> MVPISPIETVPVKLKPGMDGPKVKQWPLTEEKIKALVEICTEMEKEGKISKIGPENPYNTPVFAIKKKDSTKWRKLVDFRELNKRTQDFWEVQLGIPHPAGLKKKKSVTVLDVGDAYFSVPLDEDFRKYTAFTIPSINNETPGIRYQYNVLPQGWKGSPAIFQSSMTKILEPFKKQNPDIVIYQYMDDLYVGSDLEIGQHRTKIEELRQHLLRWGLTTPDKKHQKEPPFLWMGYELHPDKWTVQPIVLPEKDSWTVNDICKLVGKLNWASQIYPGIKVRQLSKLLRGTKALTEVIPLTEEAELELAENREILKEPVHGVYYDPSKDLIAEIQKQGQGQWTYQIYQEPFKNLKTGKYARMRGAHTNDVKQLTEAVQKITTESIVIWGKTPKFKLPIQKETWETWWTEYWQATWIPEWEFVNTPPLVKLWYQLEKEPIVGAETFYVDGAANRETKLGKAGYVTNKGRQKV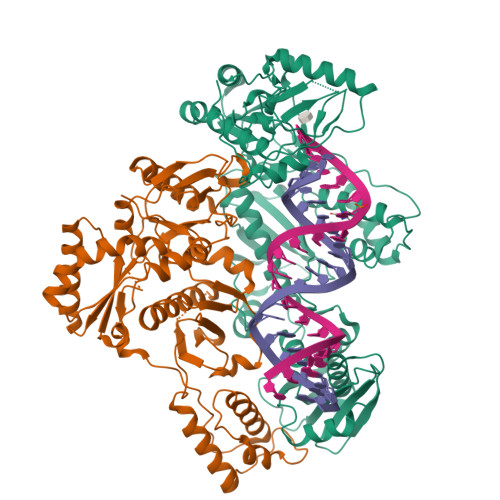VPLTNTTNQKTQLQAIYLALQDSGLEVNIVTDSQYALGIIQAQPDKSESELVNQIIEQLIKKEKVYLAWVPAHKGIGGNEQVDKLVSAGIRKIL;> MVPISPIETVPVKLKPGMDGPKVKQWPLTEEKIKALVEICTEMEKEGKISKIGPENPYNTPVFAIKKKDSTKWRKLVDFRELNKRTQDFWEVQLGIPHPAGLKKKKSVTVLDVGDAYFSVPLDEDFRKYTAFTIPSINNETPGIRYQYNVLPQGWKGSPAIFQSSMTKILEPFKKQNPDIVIYQYMDDLYVGSDLEIGQHRTKIEELRQHLLRWGLTTPDKKHQKEPPFLWMGYELHPDKWTVQPIVLPEKDSWTVNDIQKLVGKLNWASQIYPGIKVRQLSKLLRGTKALTEVIPLTEEAELELAENREILKEPVHGVYYDPSKDLIAEIQKQGQGQWTYQIYQEPFKNLKTGKYARMRGAHTNDVKQLTEAVQKITTESIVIWGKTPKFKLPIQKETWETWWTEYWQATWIPEWEFVNTPPLVKLWYQLEKEPIVGAETF> FEPTLVV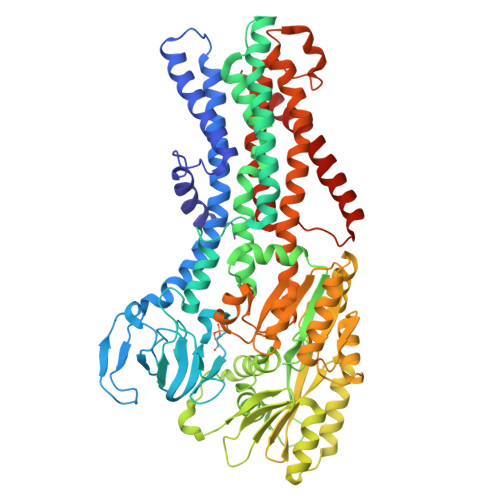QALKEAVKKLNPQAQWRNPVMFIVWIGSLLTTCISIAMASGAMPGNALFSAAISGWLWITVLFANFAEALAEGRSKAQANSLKGVKKTAFARKLREPKYGAAADKVPADQLRKGDIVLVEAGDIIPCDGEVIEGGASVDESAITGESAPVIRESGGDFASVTGGTRILSDWLVIECSVNPGETFLDRMIAMVEGAQRRKTPNEIALTILLIALTIVFLLATATLWPFSAWGGNAVSVTVLVALLVCLIPTTIGGLLSAIGVAGMSRMLGANVIATSGRAVEAAGDVDVLLLDKTGTITLGNRQASEFIPAQGVDEKTLADAAQLASLADETPEGRSIVILAKQRFNLRERDVQSLHATFVPFTAQSRMSGINIDNRMIRKGSVDAIRRHVEANGGHFPTDVDQKVDQVARQGATPLVVVEGSRVLGVIALKDIVKGGIKERFAQLRKMGIKTVMITGDNRLTAAAIAAEAGVDDFLAEATPEAKLALIRQYQAEGRLVAMTGDGTNDAPALAQADVAVAMNSGTQAAKEAGNMVDLDSNPTKLIEVVHIGKQMLMTRGSLTTFSIANDVAKYFAIIPAAFAATYPQLNALNIMCLHSPDSAILSAVIFNALIIVFLIPLALKGVSYKPLTASAMLRRNLWIYGLGGLLVPFIGIKVIDLLLTVCGLV> MINVNSTAKDIEGLESYLAN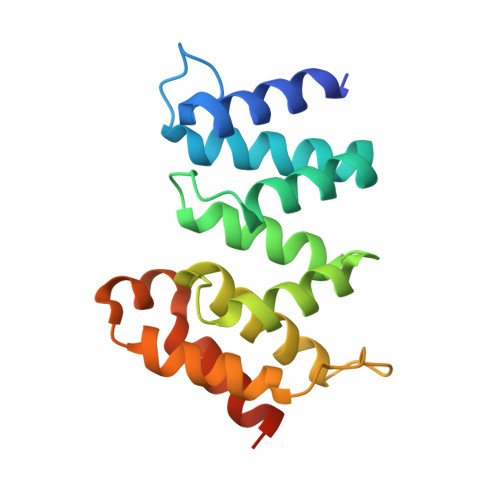GYVEANSFNDPEDDALECLSNLLVKDSRGGLSFCKKILNSNNIDGVFIKGSALNFLLLSEQWSYAFEYLTSNADNITLAELEKALFYFYCAKNETDPYPVPEGLFKKLMKRYEELKNDPDAKFYHLHETYDDFSKAYPLNNHHHHHH>[4x]SNAMKLISKNKSLLLDRSHVMGILNVTPDSFSDGGQFTHLDAALKQAEKMVKAGVSFIDIGGESTRPGAPEVSLQEELDRVLPIIEAIHQRFDTWISIDTSKAVVMEEAVKVGADLINDVRALQEPNALKVAAEANVPVCLMHMQGQPRTMQTNPSYQDLFTDISSFLSERIDACQS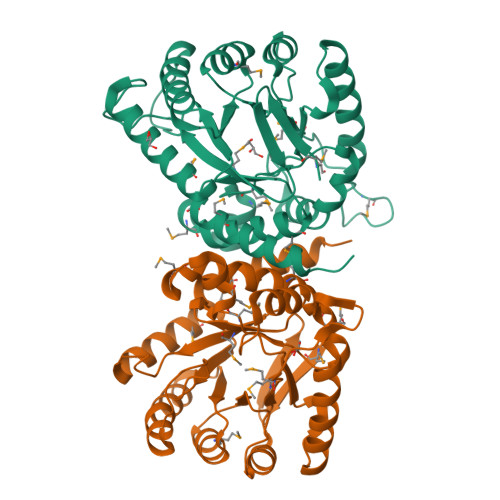VGIAKDKLILDPGFGFGKTLAHNYQLLAELERFHQFGLPLLAGMSRKSMVFKLLDVEPKMALSGSLACATIAAMKGAQIIRVHDFEQTMDIVKVCQATLEQSPH> YYDIDDVLADGTEFPCKFQYDIPGLGYLENNPGRPITKNTKLSLPLWLARILAIVGGDEALVDEEPVPFVELLPPDMFSTKVMNAIKTDPVALDLHSINSHFFSLAIKWIMLFSE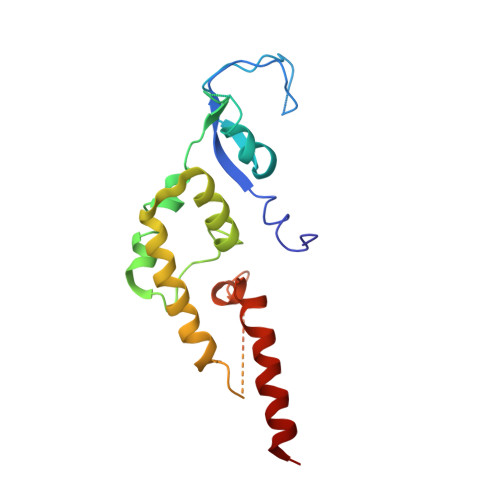KELANVVSELLLQRAQELNHHASSLSIDLNADSTGKNSANTNIATSTFLLKLEEMEKEIYKKSHESYKDTKRWMFK>MLPSTIQTLTLFLTSGGVLLSLYVSALLSYLLYSDILLKFSPTEITAPTMSLDCANASNVQAVNRSATKGVTFLLPEPEWTYPRLSCPGSTFQKALLISPHRFGETKGNSAPLIIREPFIACGPNECKHFALTHYAAQPGGYYNGTRGDRNKLRHLISVKLGKIPTVENSIFHMAAWSGSACHDGKEWTYIGVDGPDNDALLKVKYGEAYTDTYHSYANKLLRTQESACNCIGGNCYLMITDGSASGVSECRFLKIREGRIIKEIFPTGRVKHTEECTCGFASNKTIECACRDNSYTAKRPFVKLNVETDTAEIRLMCTDTYLDTPRPDDGSITGPCESNGDKGSGGIKGGFVHQRMESKIGRWYSRTMSKTERMGMGLYVKYDGDPWADSDALAFSGVMVSMKEPGWYSFGFEIKDKECDVPCIGIEMVHDGGKETWHSAATAIYCLMGSGQLLWDTVTGVDMAL[2x]

The neuraminidase inhibitors (NAIs) oseltamivir and zanamivir are the antiviral agents available in France to treat influenza A or B virus infections. The NA active site includes catalytic residues (R118, D151, R152, R224, E276, R292, R371, and Y406; N2 numbering) that interact directly with the sialic acid substrate and framework residues (E119, R156, W178, S179, D/N198, I222, E227, H274, E277, N294, and E425; N2 numbering) that stabilize the active site. NAs are divided into 3 phylogenic groups: influenza B viruses, group 1 (N1, N4, N5, and N8), and group 2 (N2, N3, N6, N7, and N9) from influenza A viruses. I221 (B NA numbering), I222 (N2 numbering), and I223 (N1 numbering) amino acids are highly conserved framework residues in NAs of influenza viruses.

We are the first to report influenza B viruses, isolated from an immunocompromised patient after prolonged oseltamivir treatment, with good fitness carrying a novel I221L substitution (B numbering) in NA that confers high-level resistance to oseltamivir. We used X-ray crystallography to understand the structural basis of resistance to oseltamivir conferred by NA carrying the I221L substitution. Crystals of the NA-I221L protein in complex with both inhibitors diffracted to high resolution, showing clearly defined density for bound oseltamivir and zanamivir. The structure of the NA-I221L-oseltamivir complex showed that the L side chain protrudes into the hydrophobic pocket of the active site that accommodates the pentyloxy substituent of oseltamivir, thus causing a change in the conformation of the inhibitor such that its C81 carbon moves about 2.2 Å from the wild-type NA bound position. Viruses isolated from an NPA collected on D34 and a nasal swab specimen collected on D40 were highly resistant to oseltamivir (IC50, 1515 and 1776 nM, respectively) and showed reduced inhibition by zanamivir (IC50, 24.3 and 27.3 nM, respectively), compared with the first wild-type isolate. The Km revealed that the I221L NA variant had a 1.9 times lower affinity for the MUNANA substrate, and the Ki values for oseltamivir carboxylate and zanamivir showed affinities that were around 84 and 51 times lower, respectively, than that for wild-type NA. In comparison to the I221T or I221V substitutions, the I221L substitution emerged in an immunocompromised patient who underwent prolonged oseltamivir treatment and conferred an increase of >100-fold in the oseltamivir IC50, a much higher fold increase than those seen for the other substitutions. In our case, I221L substitution in NA of influenza B virus isolates induced highly reduced inhibition by oseltamivir, with IC50 values greater than concentrations of oseltamivir achievable in body fluids (ie, sinus fluid, middle ear fluid, and plasma) under single and multiple dosing regimens.AMP-activated protein kinase (AMPK) is a metabolic stress-sensing kinase responsible for regulating metabolism in response to energy supply and demand. The AMPK αβγ heterotrimer comprises a catalytic α-subunit associated with β and γ regulatory subunits. Adenine nucleotides (ATP, ADP and AMP) bind interchangeably to the γ subunit where three of the four cystathionine β-synthase (CBS) tandem-repeat sequences provide nucleotide-binding sites1. The α-regulatory subunit-interacting motif 2 (αRIM2)6 is required for sensing the adenine nucleotide bound state of the γ-subunit and transducing this signal to the α-catalytic domain, resulting in either stimulation (AMP) or inhibition (ATP) of AMPK activity.

To gain further insight into the mechanism of C2-mediated AMPK activation we solved the X-ray crystal structure of full-length α2β1γ1 isoform co-crystallized with C2 and AMP to 2.99 Å resolution. The structure revealed two molecules of C2, bound within the solvent-accessible core of the γ-subunit. The phosphate groups of both C2 molecules overlap the phosphate binding sites of AMP in sites 1 and 4, while the 5-(5-hydroxyl-isoxazol-3-yl)-furan moieties occupy novel binding sites independent from the AMP-binding sites. One heterotrimer contained AMP bound at each of CBS sites 3 and 4 (white) whereas the other heterotrimer was devoid of AMP and fortuitously contained two molecules of C2 instead. In both sites the C2 molecule makes six protein-mediated hydrogen bond contacts, while C2 in γ-pSite-4 makes an additional π-stacking interaction with γ-His298. The largest structural difference between the C2 and AMP-bound heterotrimer is in the β-CBM and the N-lobe of the kinase domain, where a shift of up to 4.0 Å occurs. This shift reflects the formation of a canonical kinase salt bridge, formed between conserved residues α-Lys45 and α-Glu64, in the C2-bound heterotrimer. Strong electron density was observed for the α-RIM2 in the AMP-bound heterotrimer, but only very weak electron density was observed for α-RIM2 in the corresponding C2-bound heterotrimer and could therefore not be included in this model. Secondly, the position of C2 at γ-pSite-1 causes the side-chain guanidine group of γ-Arg70 to shift approximately 4 Å away from the AMP-bound conformation. In this new conformation, γ-Arg70 would clash with critical AMP-sensing residue α-Glu368 from the αRIM2.

>[2x]MGSSHHHHHHSQDPAEKQKHDGRVKIGHYVLGDTLGVGTFGKVKIGEHQLTGHKVAVKILNRQKIRSLDVVGKIKREIQNLKLFRHPHIIKLYQVISTPTDFFMVMEYVSGGELFDYICKHGRVEEMEARRLFQQILSAVDYCHRHMVVHRDLKPENVLLDAHMNAKIADFGLSNMMSDGEFLRTSCGSPNYAAPEVISGRLYAGPEVDIWSCGVILYALLCGTLPFDDEHVPTLFKKIRGGVFYIPEYLNRSVATLLMHMLQVDPLKRATIKDIREHEWFKQGLPSYLFPEDPSYDANVIDDEAVKEVCEKFECTESEVMNSLYSGDPQDQLAVAYHLIIDNRRIMNQASEFYLASSPPSGSFMDDSAMHIPPGLKPHPERMPPLIADSPKARCPLDALNTTKPKSLAVKKAKWHLGIRSQSKPYDIMAEVYRAMKQLDFEWKVVNAYHLRVRRKNPVTGNYVKMSLQLYLVDNRSYLLDFKSIDDEVVEQRSGSSTPQRSCSAAGLHRPRSSFDSTTAESHSLSGSLTGSLTGSTLSSVSPRLGSHTMDFFEMCASLITTLAR;>MGNTSSERAALERHGGHKTPRRDSSGGTKDGDRPKILMDSPEDADLFHSEEIKAPEKEEFLAWQHDLEVNDKAPAQARPTVFRWTGGGKEVYLSGSFNNWSKLPLTRSHNNFVAILDLPEGEHQYKFFVDGQWTHDPSEPIVTSQLGTVNNIIQVKKTDFEVFDALMVDSQKCSDVSELSSSPPGPYHQEPYVCKPEERFRAPPILPPHLLQVILNKDTGISCDPALLPEPNHVMLNHLYALSIKDGVMVLSATHRYKKKYVTTLLYKPI[2x];>MADLNWETVISSDSSPAVENEHPQETPESNNSVYTSFMKSHRCYDLIPTSSKLVVFDTSLQVKKAFFALVTNGVRAAPLWDSKKQSFVGMLTITDFINILHRYYKSALVQIYELEEHKIETWREVYLQDSFKPLVCISPNASLFDAVSSLIRNKIHRLPVIDPESGNTLYILTHKRILKFLKLFITEFPKPEFMSKSLEELQIGTYANIAMVRTTTPVYVALGIFVQHRVSALPVVDEKGRVVDIYSKFDVINLAAEKTYNNLDVSVTKALQHRSHYFEGVLKCYLHETLETIINRLVEAEVHRLVVVDENDVVKGIVSLSDILQALVLTGGEKKP[2x]>TTPSMEDYIEQIYMLIEEKGYARVSDIAEALAVHPSSVTKMV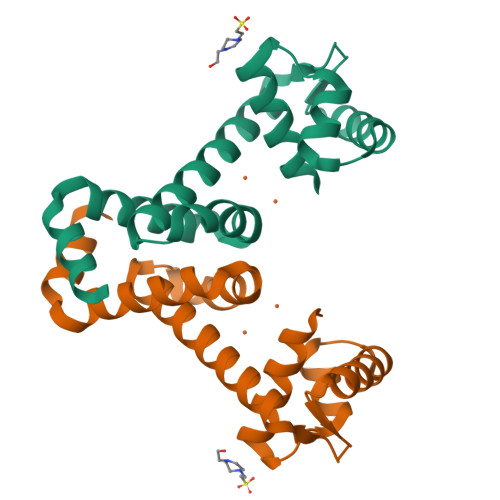QKLDKDEYLIYEKYRGLVLTSKGKKIGKRLVYRHELLEQFLRIIGVDEEKIYNDVEGIEHHLSWNSIDRIGDLVQYFEEDDARKKDLKSIQKKTEHHNQ[2x]> MRAGLLEGVIKEKGGVPVYPSYLAGEWGGSGQEIEVKSPIDLATIAKVISPSREEVERTLDVLFKRGRWSARDMPGTERLAVLRKAADIIERNLDVFAEVLVMNAGKPKSAAVGEVKAAVDRLRLAELDLKKIGGDYIPGDWTYDTLETEGLVRREPLGVVAAITPFNYPLFDAVNKITYSFIYGNAVVVKPSISDPLPAAMAVKALLDAGFPPDAIALLNLPGKEAEKIVADDRVAAVSFTGSTEVGERVVKVGGVKQYVMELGGGDPAIVLEDADLDLAADKIARGIYSYAGQRCDAIKLVLAERPVYGKLVEEVAKRLSSLRVGDPRDPTVDVGPLISPSAVDEMMAAIEDAVEKGGRVLAGGRRLGPTYVQPTLVEAPADRVKDMVLYKREVFAPVASAVEVKDLDQAIELANGRPYGLDAAVFGRDVVKIRRAVRLLEVGA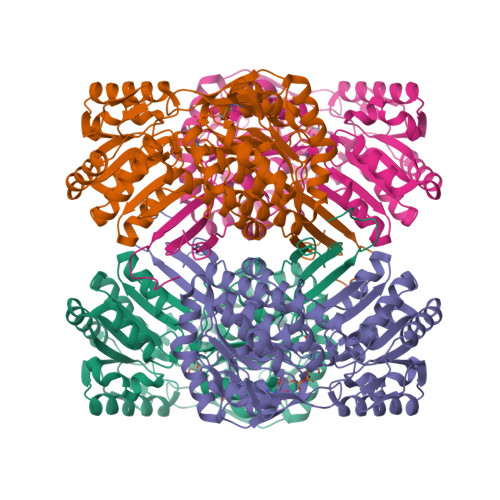IYINDMPRHGIGYYPFGGRKKSGVFREGIGYAVEAVTAYKTIVFNYKGKGVWKYE> MEPTSGFAEQPGPVKAESEEQEPAQWQALPVLSEQQSGAVELILAYAAPVLDKRQTSRLLREVSAVYPLPAQPHLKRVRPSRSAGGAQSSDLLLCLAGPSAGPRSLAELLPRPAVDPRGLGTPFLVPVPARPPLTRSQFEEARAHWPTSFHEDKQVTSALAGQLFSTQERAAMQTHMERAVCAAQRAAAQGLRAVGAVVVDPASDRVLATGHDCSSVASPLLHAVMVCIDLVAQGQGEDSLPYVCTGYDLYVTREPCVMC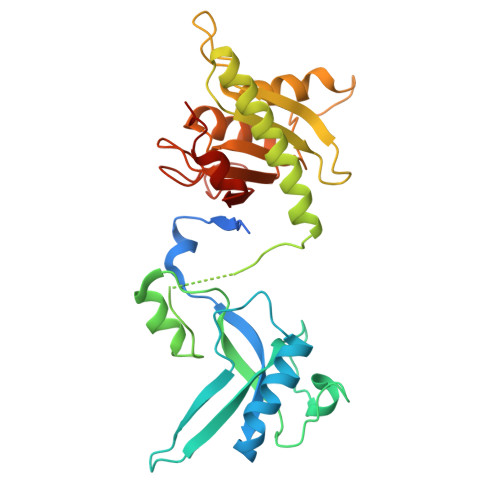AMALVHARIQRVFYGAPSPDGALGTLFRVHARPDLNHRFQVFRGILEDQCRQLDPDP>ETGTPMMPPVGVQASILSHDTIRITWADNSLPKHQKITDSRYYTVRWKTNIPANTKYKNANATTLSYLVTGLKPNTLYEFSVMVTKGRRSSTWSMTAHGATFELVPTSPPKDVTVVSKEGKPRTIIVNWQPPSEANGKITGYIIYYSTDVNAEIHDWVIEPVVGNRLTHQIQELTLDTPYYFKIQARNSKGMGPMSEAVQFRTPKADSSDKMPNDQALGSAGKGSRLP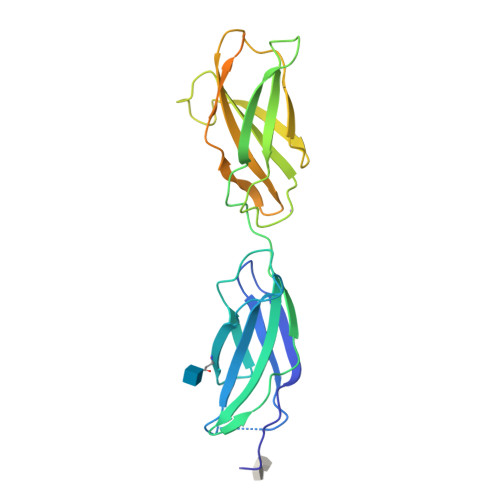DLGSDYKPPMSGSNSPHGSPTSPLDSNGTKHHHHHH[2x]>MFYDDDADLSIIQGRKVGVIGYGSQGHAHSLSLRDSGVQVRVGLKQGSRSRPKVEEQGLDVDTPAEVAKWADVVMVLAPDTAQAEIFAGDIEPNLKPGDALFFGHGLNVHFGLIKPPADVAVAMVAPKGPGHLVRRQFVDGKGVPCLVAVEQDPRGDGLALALSYAKAIGGTRAGVIKTTFK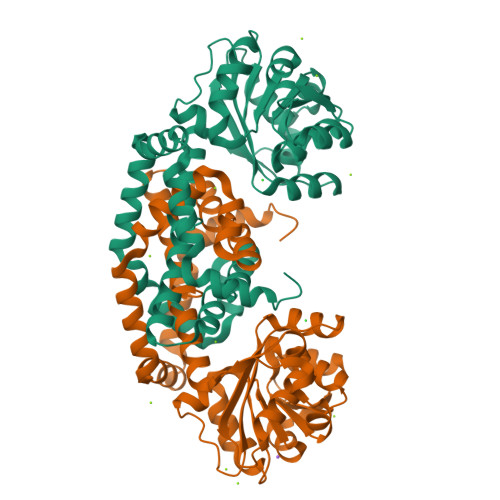DETETDLFGEQTVLCGGTEELVKAGFEVMVEAGYPAELAYFEVLHELKLIVDLMYEGGLARMYYSVSDTAEFGGYLSGPRVIDAGTKERMRDILREIQDGSFVHKLVADVEGGNKQLEELRRQNAEHPIEVVGKKLRDLMSWVDRPITETA[2x]> VTDYSGSGVKDFVFEVHRGDTTKVIGQRLKDEGVVATPSAFTDAAAGNQAIAAIQPGFYKLRTKIAGKEAVARLAEQDNRVGLLVIPEGRQLDDVSAVSNGAVTEGIFTLIARASCVDLDGDKHCVAASDLRQAATTASQGELDVPDWASNGVNAVRDDHRRIEGLIAAGRWDFDPMAEP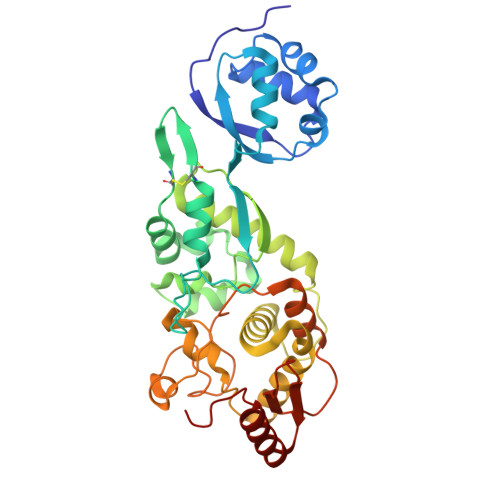EQILASLIRESNAQYQQLGLLSSDAAGLSPYQVLVVASLLQREAKPRDFAKVARVVYNRLAKHQKLEFDSTVNYPLDRQEVATTDEDRERKTLWNTYVSQGLSGTPISSPSPEALQAAERPEPGDWLYFVTIDAEGTTLFTADYNEHLANIELAKKNGILDSAR> MKIKRFGRIREVIPLPPLTEIQVESYKKALQADVPPEKRENVGIQAAFKETFPIEEGDKGKGGLVLDFLEYRIGDPPFSQDECREKDLTYQAPLYARLQLIHKDTGLIKEDEVFLGHLPLMTEDGSFIINGADRVIVSQIHRSPGVYFTPDPARPGRYIASIIPLPKRGPWIDLEVEASGVVTMKVNKRKFPLVLLLRVLGYDQETLVRELSAYGDLVQGLLDEAVLAMRPEEAMVRLFTLLRPGDPPKKDKALAYLFGLLADPKRYDLGEAGRYKAEEKLGVGLSGRTLVRFEDGEFKDEVFLPTLRYLFALTAGVPGHEVDDIDHLGNRRIRTVGELMADQFRVGLARLARGVRERMVMGSPDTLTPAKLVNSRPLEAALREFFSRSQLSQFKDETNPLSSLRHKRRISALGPGGLTRERAGFDVRDVHRTHYGRICPVETPEGANIGLITSLAAYARVDALGFIRTPYRRVKNGVVTEEVVYMTASEEDRYTIAQANTPLEGDRIATDRVVARRRGEPVIVAPEEVEFMDVSPKQVFSLNTNLIPFLEHDDANRALMGSNMQTQAVPLIRAQAPVVMTGLEERVVRDSLAALYAEEDGEVVKVDGTRIAVRYEDGRLVHPLRRYARSNQGT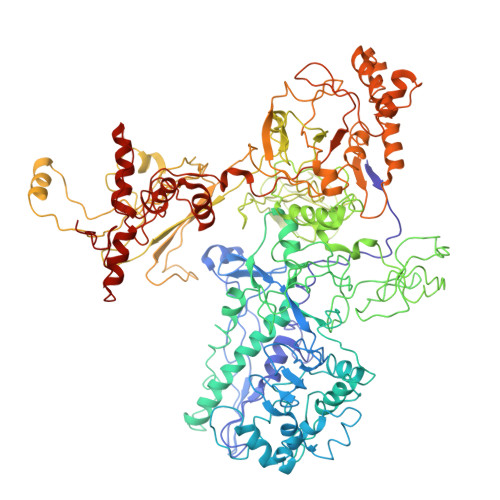AFDQRPRVRVGQRVKKGDLLADGPASEEGFLALGQNVLVAIMPFDGYNFEDAIVISEELLKRDFYTSIHIERYEIEARDTKLGPERITRDIPHLSEAALRDLDEEGIVRIGAEVKPGDILVGRTSFKGEQEPSPEERLLRSIFGEKARDVKDTSLRVPPGEGGIVVGRLRLRRGDPGVELKPGVREVVRVFVAQKRKLQVGDKLANRHGNKGVVAKILPVEDMPHLPDGTPVDVILNPLGVPSRMNLGQILETHLGLAGYFLGQRYISPVFDGATEPEIKELLAEAFNLYFGKRQGEGFGVDKREKEVLARAEKLGLVSPGKSPEEQLKELFDLGKVVLYDGRTGEPFEGPIVVGQMFIMKLYHMVEDKMHARSTGPYSLITQQPLGGKAQFGGQRFGEMEVWALEAYGAAHTLQEMLTIKSDDIEGRNAAYQAIIKGEDVPEPSVPESFRVLVKELQALALDVQTLDEKDNPVDVFEGLASKR>MRLINLDGRIHLVTGDGVVDVAKASEQRFGPDPQDLYQHWDAFQEWARTAALPAPSARVGTIGSPAPLPRQVFAVGLNYDDHATESGLSKPEHPVIFTKFVSSITGPVETVQLPAGSVDWEVELVVVMGRGGRNIPEDRAWEFVAGVSVGQDLSERDLQLAGPAPQFSLAKSHAGFSPIGPELVTVDELPDPDDLELGAEINGETVQHSRTSQLIFPVSNLIAYLSDTVELYPGDVIFTG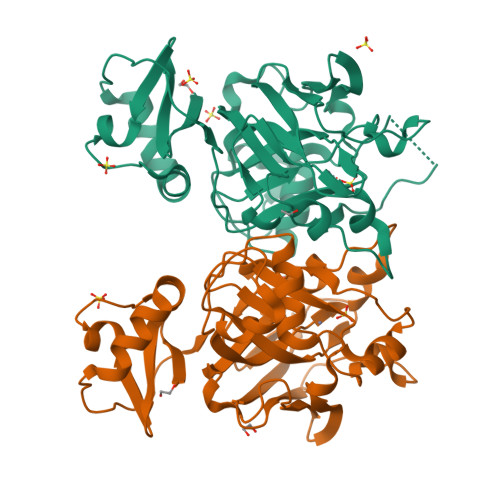TPSGVGMGRNPKRFLAPGDELRTYITGVGEFTQRFVTADSASVAPRSGHHHHHH[2x]> FNGSETDVECFLGRAACVHVTEIQNKDATGIDNHREAKLFNDWKINLSSLVQLRKKLELFTYVRFDSEYTILATA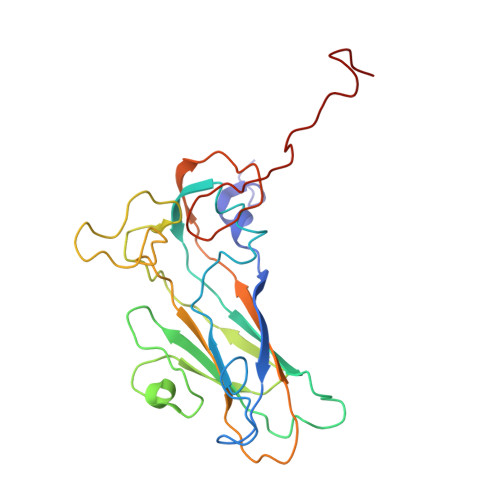SQPDSANYSSNLVVQAMYVPPGAPNPKEWDDYTWQSASNPSVFFKVGDTSRFSVPYVGLASAYNCFYDGYSHDDAETQYGITVLNHMGSMAFRIVNEHDEHKTLVKIRVYHRAKHVEAWIPRAPRALPYTSIGRTNYPKNTEPVIKKRKGDIKSY>METNVTAAAPSDHPVFVLVHGAWHGAWCYAHVAAALAERGYLSIARDLPAHGINARFPASYLERPLDKDAFGAEPSPVAN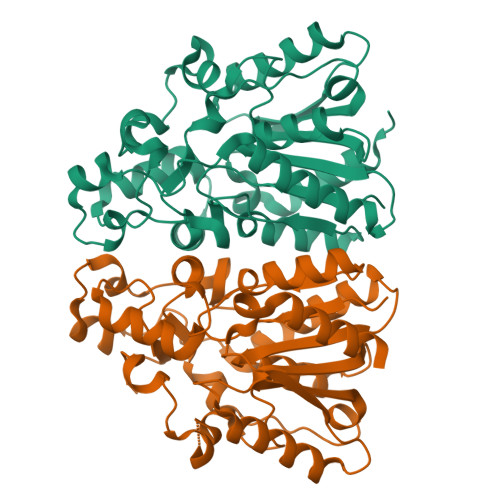TTLDDYATQVMEAVDDAYALGHGKVVLVGHSMGGLAITAAAERAPEKIAKIVYLAAFMPASGVPGLDYVRAPENKGEMLAPLMLASPRVAGALRIDPRSGDAAYRALAKRALYDDAAQADFEAMANLMTCDVPAAPFATAIPTTAARWGAIDRHYIKCLADRVILPALQQRFIDEADAFVPGNPTHVHQLDSSHSPFVSQPGVLAGVLVDIAKSIALEHHHHHH[3x]>HHHHHHSSGLVPRGSHMMSLLSKTRELNTLLQKHKGIAVDFKDVAQTISSVTVTNVFIVSRRGKILGSSLNELLKSQRIIQMLEERHIPSEYTERLMEVKQTESNIDIDNVLTVFPPENRELFIDSRTTIFPILGGGERLGTLVLGRVHDDFNENDLVLGEYAATVIGMEILREKHSEVEKEAR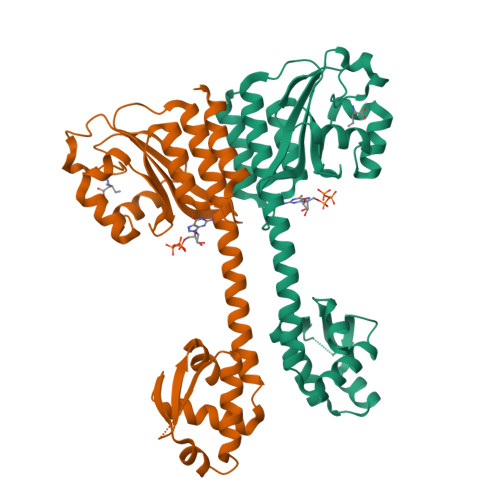DKAAITMAINSLSYSEKEAIEHIFEELGGTEGLLIASKVADRVGITRSVIVNALRKLESAGVIESRSLGMKGTFIKVKKEKFLDELEKSK[2x]5'-O-[(2-phenylethyl)carbamoyl]guanosine | C19 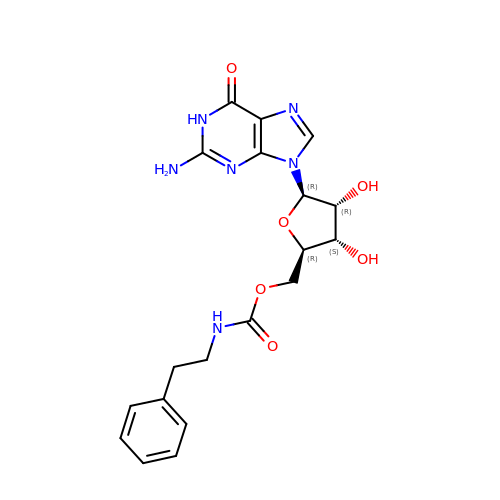H22 N6 O6 | QOLMNPPGFSBCCF-LSCFUAHRSA-N>[2x]MHHHHHHAAGIPMNNPAIKRIGNHITKSPEDKREYRGLELANGIKVLLISDPTTDKSSAALDVHIGSLSDPPNIAGLSHFLQHMLFLGTKKYPKENEYSQFLSEHAGSSNAFTSGEHTNYYFDVSHEHLEGALDRFAQFFLSPLFDESAKDREVNAVDSEHEKNVMNDAWRLFQLEKATGNPKHPFSKFGTGNKYTLETRPNQEGIDVRQELLKFHSAYYSSNLMAVVVLGRESLDDLTNLVVKLFSEVENKNVPLPEFPEHPFQEEHLKQLYKIVPIKDIRNLYVTFPIPDLQKYYKSNPGHYLGHLIGHEGPGSLLSELKSKGWVNTLVGGQKEGARGFMFFIINVDLTEEGLLHVEDIILHMFQYIQKLRAEGPQEWVFQELKDLNAVAFRFKDKERPRGYTSKIAGILHYYPLEEVLTAEYLLEEFRP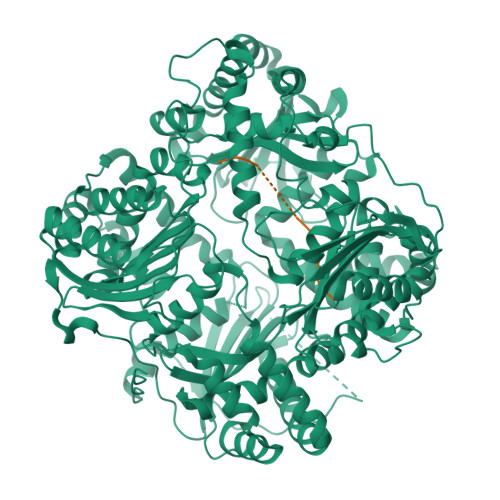DLIEMVLDKLRPENVRVAIVSKSFEGKTDRTEEWYGTQYKQEAIPDEVIKKWQNADLNGKFKLPTKNEFIPTNFEILPLEKEATPYPALIKDTAMSKLWFKQDDKFFLPKANLNFEFFSPFAYVDPLHSNMAYLYLELLKDSLNEYAYAAELAGLSYDLQNTIYGMYLSVKGYNDKQPILLKKIIEKMATFEIDEKRFEIIKEAYMRSLNNFRAEQPHQHAMYYLRLLMTEVAWTKDELKEALDDVTLPRLKAFIPQLLSRLHIEALLHGNITKQAALGIMQMVEDTLIEHAHTKPLLPSQLVRYREVQLPDRGWFVYQQRNEVHNNSGIEIYYQTDMQSTSENMFLELFAQIISEPAFNTLRTKEQLGYIVFSGPRRANGIQGLRFIIQSEKPPHYLESRVEAFLITMEKSIEDMTEEAFQKHIQALAIRRLDKPKKLSAESAKYYGEIISQQYNFDRDNTEVAYLKTLTKEDIIKFYKEMLAVDAPRRHKVSVHVLAREMDSCPVVGEFPCQNDINLSQAPALPQPEVIQNMTEFKRGLPLFPLVKPHINFMAAKL;>AYRPSETLCGGELVDTLQFVCGDRGFYFSRPASRVSRRSRGIVEECCFRSCDLALLETYCATPAKSE[2x]>[2x]MDEGMWLMQQLGRKYAQMKERGLKMKEYDLYNPNGTSLKDAVVLFDGGCTGEVVSD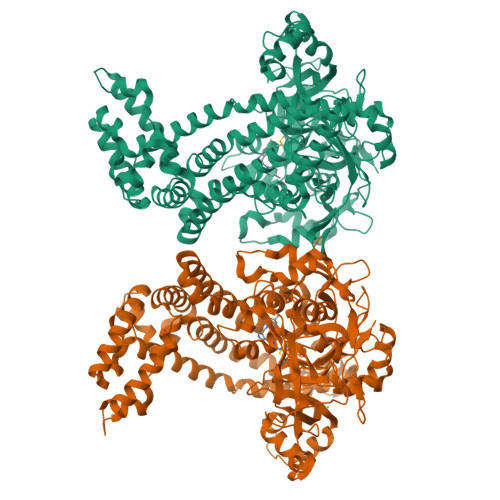RGLVLTNHHCGYDMIQAHSTLEHNYLENGFWAMREADELPNKDISVVFIDKIEDVTDYVKKELKAIKDPNSMDYLSPKYLQKLADKKAGKNFSAKNPGLSVEIKAFYGGNLYLMFTKKTYTDVRLVGAPPSSIGKFGADTDNWIWPRHTGDFSIFRIYADKNGNPAPYSEDNVPLKPKRFFNISLGGVQENDYAMIMGFPGTTHRYFTASEVDEWKSIDNDIRIRMRDIRQGVMLREMLADPQIKIMYSAKYAASQNAYKRAIGANWAIKTRGLRQNKQAMQDRLIAWGAKQGTPRYEEAVHEIDATVAKRADLRRRYWMIEEGIIRGIEFARSPIPTEDETKALQGNDASARKEAIDKIRTRYSKFANKDYSAEVDKKVAVAMLTEYLKEIPYENLPLHLRLVKDRFAGDVQAYVDDIFARSVFGSEAQFDAFAAVPSVEKLAEDPMVLFASSVFDEYRKLYNELRPYDDPILRAQRTYIAGLLEMDGDQDQFPDANLTLRFTYGQVKGYSPRDNVYYGHQTTLDGVMEKEDPDNWEFVVDPKLKAVYERKDFGRYADRSGRMPVAFCATTHTTGGNSGSPVMNANGELIGLNFDRNWEGVGGDIQYLADYQRSIIVDIRYVLLVIDKVGGCQRLLDEMNIVPAHHHHHH> GGCUUAUCAAGAGAGGGUGAGCGACUGGCGCGAAGACCCCCGGCAACCAGAAAUGGUGCCAAUUCCUGCAGCGGAA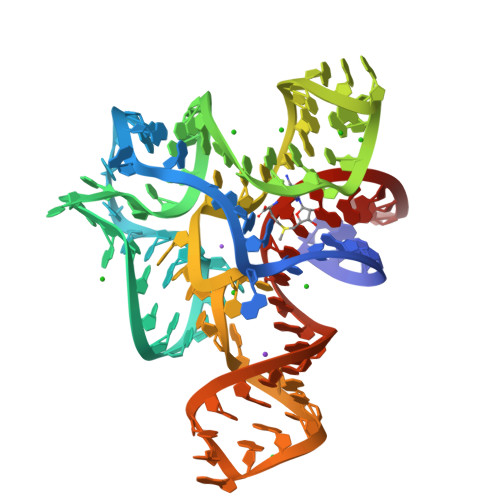ACGUUGAAAGAUGAGCCG>[2x]TRDRVPTYQYNMNFEKLGKCIIINNKNFDKVTGMGVRNGTDKDAEALFKCFRSLGFDVIVYNDCSCAKMQDLLKKASEEDHTNAACFACILLSHGEENVIYGKDGVTPIKDLTAHFRGARCKTLLEKPKLFFIQAARGTELDDGIQADSGPIN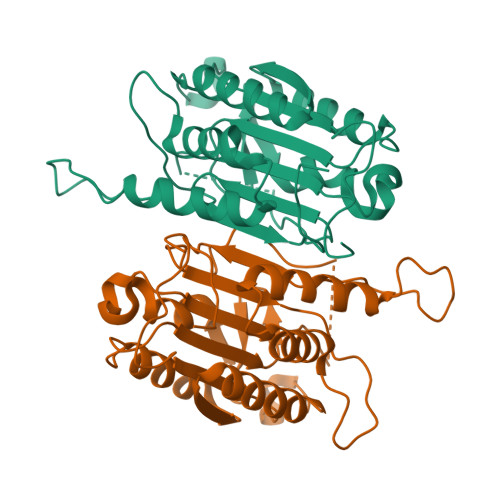DTDANPRYKIPVEADFLFAYSTVPGYYSWRSPGRGSWFVQALCSILEEHGKDLEIMQILTRVNDRVARHFESQSDDPHFHEKKQIPCVVSMLTKELYFSQ> SNAEMAVEDKEKQQEERVYQLLPKGDVEGMRELHQRGMSFSPYEPTGIYVKPDEEVVIQVEGTQQIKAYIGTYSYEKEGPKQFNLHPGENKISSSNGGLLYFYNYH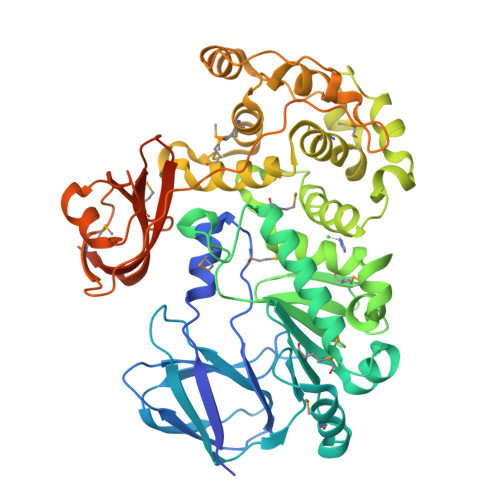NTGEVVAKVKKGGTPNPLFILGKHTTKDWKRMLAENPDPYAIEMKGENSLLTMHPETVAEHLKQEDPAALLKKHDEIINIEHKMSGLSKDGAGVANQGKHSIHFVEDWYTDDYMYATYYRTAYSKGNLESVLNLEELTNDGWGPWHEVGHQHQQDTWLWDGLGEVTVNIYSLAVQTTFGHKTRLEQEGRYEAAFAYLGKPDAQEKMNEFEKLVMFWQLHLAYGDQFYPNLHQMYRLLHDTELPKSDEEKKQMFIYMTSKVAGQNLIPFFDKWGLSANDATREKIEKLNLPKLEKEIWLSTDSNPIREKQIELYEAPYGEPNNEKIQNMVIGTTYDEEKAKELVQNLGEGVKTTGVIMQDTPEVGEKTVKVEIVDGKGNKNFIPVVVNVGYGDSLLVYGLNYTWGGLEVNRNSTSWYENI Here, a method for presenting crystals of soluble and membrane proteins growing in the lipid cubic or sponge phase for in situ diffraction data collection at cryogenic temperatures is introduced. The method is a variant on the recently introduced in meso in situ serial crystallography (IMISX) method that enables crystallo­graphic measurements at cryogenic temperatures where crystal lifetimes are enormously enhanced whilst reducing protein consumption dramatically. The new approach has been used to generate high-resolution crystal structures of a G-protein-coupled receptor, α-helical and β-barrel transporters and an enzyme as model integral membrane proteins. Insulin and lysozyme were used as test soluble proteins.

The first protein used for this purpose was AlgE, an alginate transporter that resides in the outer membrane of P. aeruginosa. Because the crystal used for data collection was long (150 µm), it was possible to collect all of the required data from four separate locations on the one crystal in the IMISX well. 20–30° of data were combined from the four sites to give a total of 100° of data. The crystals, which belonged to space group P212121, diffracted to 2.4 Å resolution with a completeness of 90.8%, a CC1/2 of 0.62 and an 〈I/σ(I)〉 of 1.45 in the highest resolution shell. The corresponding electron-density map was of high quality and the model was similar (backbone r.m.s.d. of 0.599 Å over 403 residues) to that obtained using crystals harvested from IMISX plates with data collected at 100 K, where the resolution was 2.9 Å. The data-quality and refinement statistics were comparable between IMISXcryo data and the previously published IMISX data obtained from 175 crystals at RT. Dimannuronate, a surrogate for the alginate polysaccharide transported by AlgE, was included with the protein during crystallogenesis. The expectation was that it would bind in the electrostatic pore midway across the β-barrel through which alginate is proposed to pass en route to the extracellular space. However, density for two MES buffer molecules was clearly visible.

> MNSSRSVNPRPSFAPRALSLAIALLLGAPAFAANSGEAPKNFGLDVKITGESENDRDLGTAPGGTLNDIGIDLRPWAFGQWGDWSAYFMGQAVAATDTIETDTLQSDTDDGNNSRNDGREPDKSYLAAREFWVDYAGLTAYPGEHLRFGRQRLREDSGQWQDTNIEALNWSFETTLLNAHAGVAQRFSEYRTDLDELAPEDKDRTHVFGDISTQWAPHHRIGVRIHHADDSGHLRRPGEEVDNLDKTYTGQLTWLGIEATGDAYNYRSSMPLNYWASATWLTGDRDNLTTTTVDDRRIATGKQSGDVNAFGVDLGLRWNIDEQWKAGVGYARGSGGGKDGEEQFQQTGLESNRSNFTGTRSRVHRFGEAFRGELSNLQAATLFGSWQLREDYDASLVYHKFWRVDDDSDIGTSGINAALQPGEKDIGQELDLVVTKYFKQGLLPASMSQYVDEPSALIRFRGGLFKPGDAYGPGTDSTMHRAFVDFIWRF> MAKSLPLNSRSKTTALKQPRELFSYARDIDGKYVYDDPENSLSYYYLPDSTIDTGIDLQGGYSKFKKIPDEQNLADFNSLLKAIIKYETSEGKKISSDIITFREIMTKILSLPYNLTDPIDLYVVPFDGQLFIKSDDELDMKRRKEQEVRMKQTNTVERYDYMKRCEYVGYKFETIATIPKPWSQVSRSQIENRNKKVVNNYEQYLSVIRTGIGNVKLVLAGEIDCCWDYLPDEQNKKLNHYVELKTSRIIENNSQVVSFEQKLFKAWCQCFLMGVTKIIYGFRDNNLILKNVELFNTEEIPILIKNNPLTNAATEKKINCTNALKWYGAVVDWLNTTVDKKDEIKSYRLKYDPVRKSFTLSETDSETNEKLRNGQLLTPEFTEWRQSLKK

Rai1 homologs share several highly conserved sequence motifs, and our structural studies show that they are located in the active site region, mediating the binding of the divalent metal ions and/or the RNA. We have found substantial variations in the activity profiles of the Rai1 homologs, and discovered that some of them possess a new 5′ triphosphonucleotide hydrolase (TPH) activity. The overall structures of CaRai1, AgRai1 and SsRai1 are similar to those of SpRai1 (16), KlDxo1 (18), and MmDXO. Each structure contains two mixed β-sheets that are surrounded by α-helices.

There are essentially no conformational changes in CaRai1 upon RNA binding, with rms distance of 0.38 Å for the Cα atoms of the two structures. The structures of the AgRai1 and CaRai1 free enzymes will not be described further here. CaRai1 had very low activity in our biochemical assays except for decapping toward unmethylated RNA. The CaRai1 and SsRai1 structures are especially similar, consistent with the 58% sequence identity between them. The αC helix is absent in AgRai1 but contains more than four turns in CaRai1 and SsRai1, which also have a longer αD helix.> GSHMDASVMSTTYALSAAQTEIWLAQQLYPDSPVYNIAQYTVIEGVIEPAVFEAALRQVIDEADTLRLQFIDSDDGLRQRIGTPAWSMPVLDLTAQADPQAAAQAWMRADYQQPVNLTQGPLFCYALLKVAPAQWMWYQRYHHIMMDGYGAYLIAQRVAYVYSALCEGTTPAECDFGSILQLLE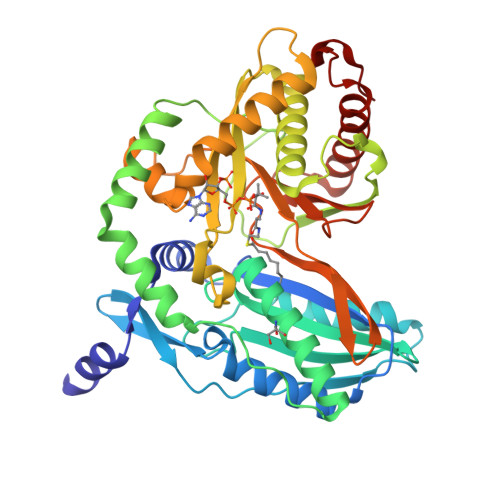SDAQYQISAQRAQDEAYWLKHCANWSEPATLASRSAPVLQQRLRQTTYLAIQALGDTAPDARRLAQFMTAAMAAYLYRFTGEQDVVLGLPVKVRFGADRHIPGMKSNTLPLRLTMRPGMNLSSLMQQAAQEMQSGLRHQRYPSEALRRQLGMPSGQRLFGTTVNVMPFDLDLSFGGYSATNHNLLNGPAEDLMLGVYWTPGSHQLRIDFDANPACYTPEGLGAHQRRFIRFMQVLAADATQPIDSIDLLD> ATIKDVAKRANVSTTTVSHVINKTRFVAEETRNAVWAAIKELHYSPSAVARSLKVNHTKSIGLLATSSEAAYFAEIIEAVEKNCFQKGYTLILGNAWNNLEKQRAYLSMMAQKRVDGLLVMCSEYPEPLLAMLEEYRHIPMVVMDAGEAKADFTDAVIDNAFEGGYMAGRYLIERGHREIGVIPGPLERNTGAGRLAGFMKAMEEAMIKVPESWIVQGDFEPESGYRAMQQILSQPHRPTAVFCGGDIMAMGALCAADEMGLRVPQDVSLIGYDNVRNA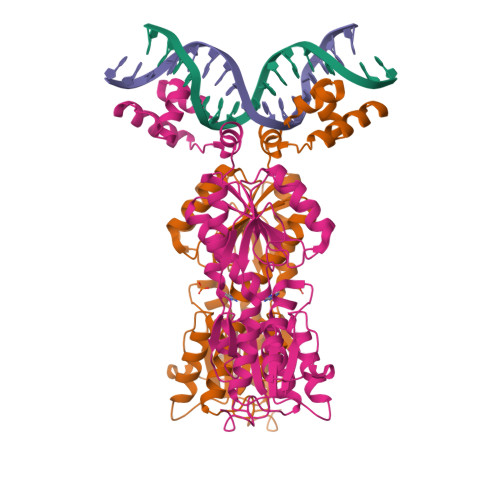RYFTPALTTIHQPKDSLGETAFNMLLDRIVNKREEPQSIEVHPRLIERRSVADGPFRDYRR3-[5-chloranyl-6-[(1~{R})-1-pyridin-2-ylethoxy]-1,2-benzoxazol-3-yl]propanoic acid | C17 H15 Cl N2 O4 | 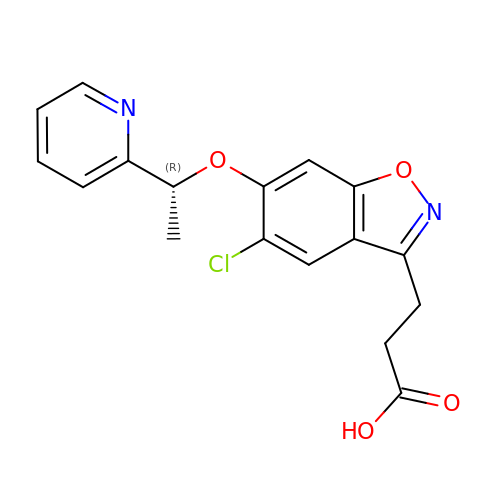WPAHVUADNLXSOM-SNVBAGLBSA-N>SMLQSMAAQRQRALAIMCRVFVGSIYYELGEDTIRQAFAPFGPIKSIDMSWDSVTMKHKGFAFVEYEVPEAAQLALEQMNSVMLGGRNIKVGRPSNIGQAQPIIDQ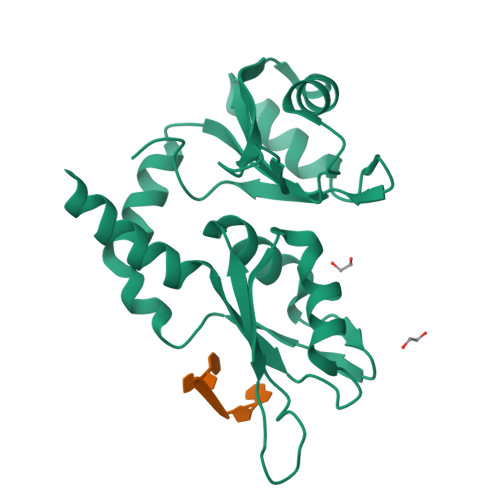LAEEARAFNRIYVASVHQDLSDDDIKSVFEAFGKIKSCTLARDPTTGKHKGYGFIEYEKAQSSQDAVSSMNLFDLGGQYLRVGKAVTPPMP[2x]>NTSLEAIVQNASSDNQGIQLSAVQAARKLLSSDRNPPIDDLIKSGILPILVHCLERDDNPSLQFEAAWALTNIASGTSEQTQAVVQSNAVPLFLRLLHSPHQNVCEQAVWALGNIIGDGPQCRDYVISLGVVKPLLSFISPSIPITFLRNVTWVMVNLCRHKDPPPPMETIQEILPALCVLIHHTDVNILVDTVWALSYLTDAGNEQIQMVIDSGIVPHLVPLLSHQEVKVQTAALRAVGNIVTGTDEQTQVVLNCDALSHFPALLTHPKEKINKEAVWFLSNITAGNQQQVQAVIDANLVPMIIHLLDKGDFGTQKEAAWAISNLTISGRKDQVAYLIQQNVIPPFCNLLTVKDAQVVQVVLDGLSNILKMAEDEAETIGNLIEECGGLEKIEQLQNHENEDIYKL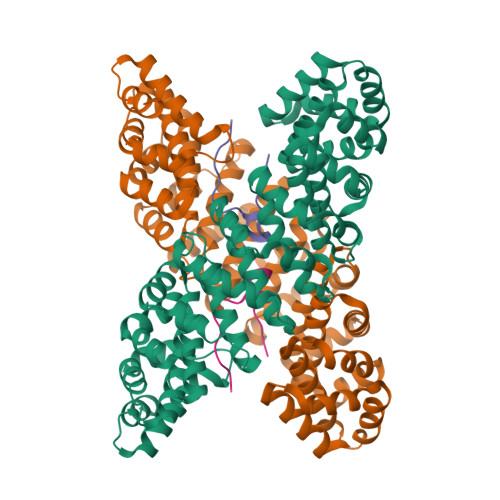AYEIIDQFF[2x];>SGKRKLITSEEERSPAKRGRKS[2x]>MGSSHHHHHHENLYFQSNAGPSIEVYVSAVSSPSRFWVQFVGPQVAQLDDLVAHMTEYYSKKENREAHTLRHVSVGQVVAAVFRHDGRWYRARVHDIRPNEFDSSQQVADVFYLDYGDSEYVATHELCELRADLLRLRFQAMECF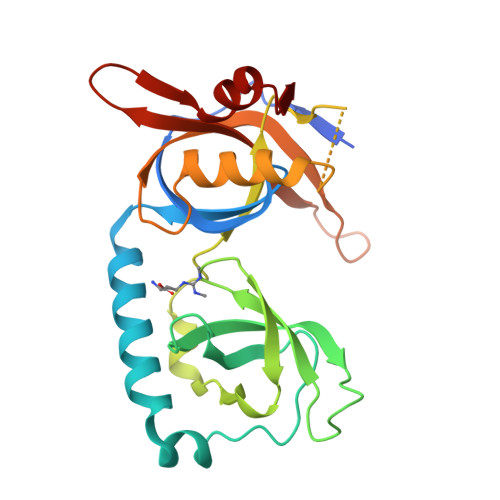LAGVRPASGEEAVSPSGQRWDKWHPQAVERFEELTQVARWKALVSRTCTYKKTATAEGEKDKEIPGIKLFDVTDEGELDVGAVLVAEGWAVA[2x]> GPLGSPEFMALAVAPWGRQWEEARALGRAVRMLQRLEEQCVDPRLSVSPPSLRDLLPRTAQLLREVAHSRRAAGGGGPGGPGGSGDFLLIYLANLEAKSRQVAALLPPRGRRSANDELFRAGSRLRRQLAKLAIIFSHMHAELHALFPGGKYCGHMYQLTKAPAHTFWRESCGARCVLPWAE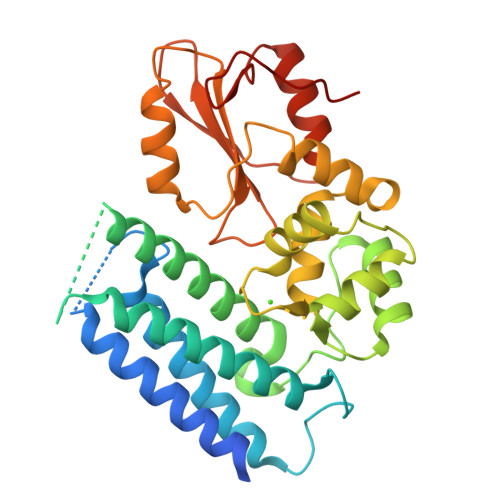FESLLGTCHPVEPGCTALALRTTIDLTCSGHVSIFEFDVFTRLFQPWPTLLKNWQLLAVNHPGYMAFLTYDEVQERLQACRDKPGSYIFRPSCTRLGQWAIGYVSSDGSILQTIPANKPLSQVLLEGQKDGFYLYPDGKTHNPDLTELG> MTSAEMTSPNNNSEHQAIAKMRTMIEGFDDISHGGLPIGRSTLVSGTSGTGKTLFSIQFLYNGIIEFDEPGVFVTFEETPQDIIKNARSFGWDLAKLVD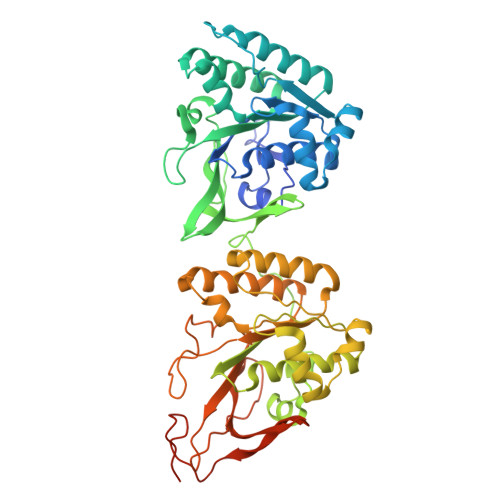EGKLFILDASPDPEGQEVVGGFDLSALIERINYAIQKYRARRVSIDSVTSVFQQYDASSVVRRELFRLVARLKQIGATTVMTTERIEEYGPIARYGVEEFVSDNVVILRNVLEGERRRRTLEILKLRGTSHMKGEYPFTITDHGINIFPLGAMRLTQRSSNVRVSSGVVRLDEMCGGGFFKDSIILATGATGTGKTLLVSRFVENACANKERAILFAYEESRAQLLRNAYSWGMDFEEMERQNLLKIVCAYPESAGLEDHLQIIKSEINDFKPARIAIDSLSALARGVSNNAFRQFVIGVTGYAKQEEITGLFTNTSDQFMGAHSITDSHISTITDTIILLQYVEIRGEMSRAINVFKMRGSWHDKAIREFMISDKGPDIKDSFRNFERIISGSPTRITVDEKSELSRIVRGVQEKGPES> MVANQANLIDNKRELEQHALVPYAQGKSIHQLFEEQAEAFPDRVAIVFENRRLSYQELNRKANQLARALLEKGVQTDSIVGVMMEKSIENVIAILAVLKAGGAYVPIDIEYPRDRIQYILQDSQTKIVLTQKSVSQLVHDVGYSGEVVVLDEEQLDARETANLHQPSKPTDLAYVIYTSGTTGKPKGTMLEHKGIANLQSFFQNSFGVTEQDRIGLFASMSFDASVWEMFMALLSGASLYILSKQTIHDFAAFEHYLSENELTIITLPPTYLTHLTPERITSLRIMITAGSASSAPLVNKWKDKLRYINAYGPTETSICATIWEAPSNQLSVQSVPIGKPIQNTHIYIVNEDLQLLPTGSEGELCIGGVGLARGYWNRPDLTAEKFVDNPFVPGEKMYRTGDLAKWLTDGTIEFLGRIDHQVKIRGHRIELGEIESVLLAHEHITEAVVIAREDQHAGQYLCAYYISQQEATPAQLRDYAAQKLPAYMLPSYFVKLDKMPLTPNDKIDRKALPEPDLTANQSQAAYHPPRTETESILVSIWQNVLGIEKIGIRDNFYSLGGDSIQAIQVVARLHSYQLKLETKDLLNYPTIEQ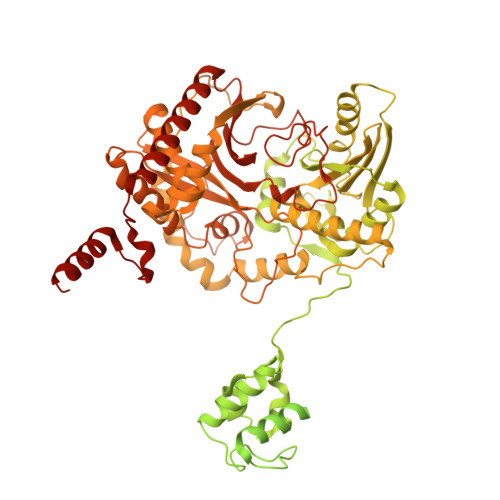VALFVKSTTRKSDQGIIAGNVPLTPIQKWFFGKNFTNTGHWNQSSVLYRPEGFDPKVIQSVMDKIIEHHDALRMVYQHENGNVVQHNRGLGGQLYDFFSYNLTAQPDVQQAIEAETQRLHSSMNLQEGPLVKVALFQTLHGDHLFLAIHHLVVDGISWRILFEDLATGYAQALAGQAISLPEKTDSFQSWSQWLQEYANEADLLSEIPYWESLESQAKNVSLPKDYEVTDCKQKSVRNMRIRLHPEETEQLLKHANQAYQTEINDLLLAALGLAFAEWSKLAQIVIHLEGHGREDIIEQANVARTVGWFTSQYPVLLDLKQTAPLSDYIKLTKENMRKIPRKGIGYDILKHVTLPENRGSLSFRVQPEVTFNYLGQFDADMRTELFTRSPYSGGNTLGADGKNNLSPESEVYTALNITGLIEGGELVLTFSYSSEQYREESIQQLSQSYQKHLLAIIAHCTEKKEVERTPSDFSVKGLQMEEMDDIFELLANRLRGSRSHHHHHH> AMVSVSGIRKVQRAEG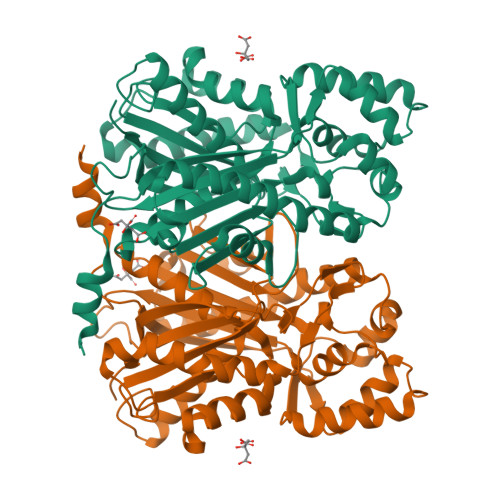PATVLAIGTANPPNCVDQSTYADYYFRVTNSEHMTDLKKKFQRICERTQIKNRHMYLTEEILKENPNMCAYKAPSLDAREDMMIREVPRVGKEAATKAIKEWGQPMSKITHLIFCTTSGVALPGVDYELIVLLGLDPSVKRYMMYHQGCFAGGTVLRLAKDLAENNKDARVLIVCSENTSVTFRGPSETDMDSLVGQALFADGAAAIIIGSDPVPEVENPLFEIVSTDQQLVPNSHGAIGGLLREVGLTFYLNKSVPDIISQNINDALSKAFDPLGISDYNSIFWIAHPGGRAILDQVEEKVNLKPEKMKATRDVLSNYGNMSSACVFFIMDLMRKKSLEAGLKTTGEGLDWGVLFGFGPGLTIETVVLRSMAI> MHHHHHHHAVRASEISRVYEAYPEKKATLYFLVLGFLALIVGSLFGPFQALNYGNVDAYPLLKRLLPFVQSYYQGLTLHGVLNAIVFTQLFAQAIMVYLPARELNMRPNMGLMWLSWWMAFIGLVVFALPLLANEATVLYTFYPPLKGHWAFYLGASVFVLSTWVSIYIVLDLWRRWKAANPGKVTPLVTYMAVVFWLMWFLASLGLVLEAVLFLLPWSFGLVEGVDPLVARTLFWWTGHPITYFWLLPAYAIIYTILPKQAGGKLVSDPMARLAFLLFLLLSTPVGFHHQFADPGIDPTWKMIHSVLTLFVAVPSLMTAFTVAASLEFAGRLRGGRGLFGWIRALPWDNPAFVAPVLGLLGFIPGGAGGIVNASFTLDYVVHNTAWVPGHFHLQVASLVTLTAMGSLYWLLPNLTGKPISDAQRRLGLAVV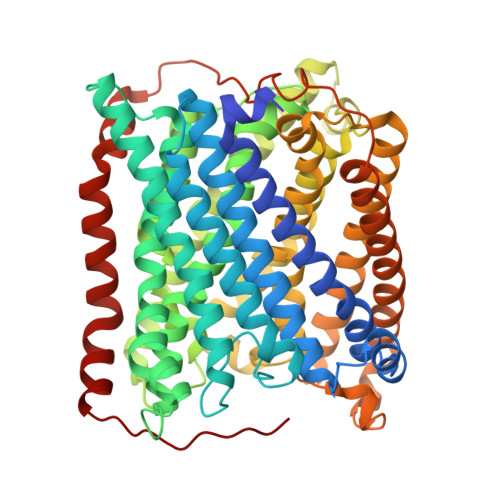WLWFLGMMIMAVGLHWAGLLNVPRRAYIAQVPDAYPHAAVPMVFNVLAGIVLLVALLLFIYGLFSVLLSRERKPELAEAPLPFAEVISGPEDRRLVLAMDRIGFWFAVAAILVVLAYGPTLVQLFGHLNPVPGWRLW>GSVPATLPQLTP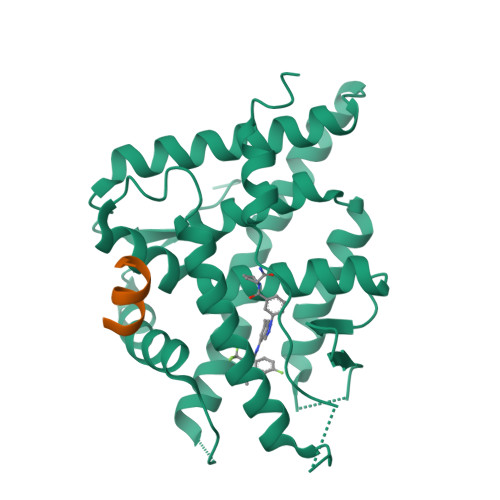TLVSLLEVIEPEVLYAGYDSSVPDSTWRIMTTLNMLGGRQVIAAVKWAKAIPGFRNLHLDDQMTLLQYSWMYLMAFALGWRSYRQSSANLLCFAPDLIINEQRMTLPGMYDQCKHMLYVSSELHRLQVSYEEYLCMKTLLLLSSVPKDGLKSQELFDEIRMTYIKELGKAIVKREGNSSQNWQRFYQLTKLLDSMHEVVENLLNYCFQTFLDKTMSIEFPEMLAEIITNQIPKYSNGNIKKLLFHQK[3x];>[3x]KENALLRYLLDK> GAMQNNNEFKIGNRSVGYNHEPLIICEIGINHEGSLKTAFEMVDAAYNAGAEVVKHQTHIVEDEMSDEAKQVIPGNADVSIYEIMERCALNEEDEIKLKEYVESKGMIFISTPFSRAAALRLQRMDIPAYKIGSGECNNYPLIKLVASFGKPIILSTGMNSIESIKKSVEIIREAGVPYALLHCTNIYPTPYEDVRLGGMNDLSEAFPDAIIGLSDHTLDNYACLGAVALGGSILER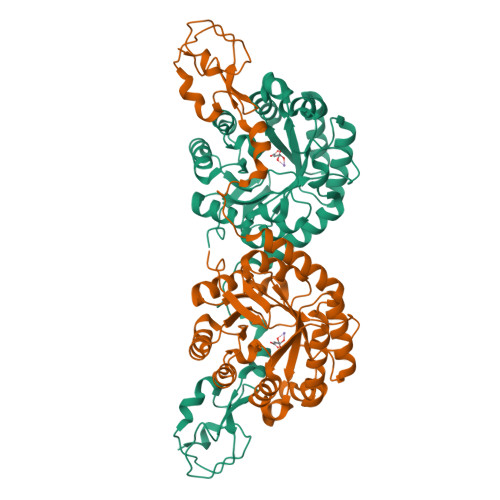HFTDRMDRPGPDIVCSMNPDTFKELKQGAHALKLARGGKKDTIIAGEKPTKDFAFASVVADKDIKKGELLSGDNLWVKKPGNGDFSVNEYETLFGKVAACNIRKGAQIKKTDIE>SKGLEDSSTISFITWNIDGLDGCNLPERARGVCSCLALYSPDVVFLQEVIPPYCAYLKKRAASYTIITGNEEGYFTAILLKKGRVKFKSQEIIPFPNTKMMRNLLCVNVSLGGNEFCLMTSHLESTREHSAERIRQLKTVLGKMQEAPDSTTVIFA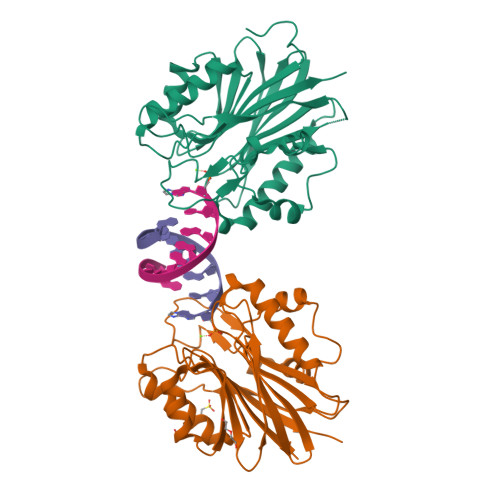GDTNLRDQEVIKCGGLPDNVFDAWEFLGKPKHCQYTWDTKANNNLRIPAAYKHRFDRIFFRAEEGHLIPQSLDLVGLEKLDCGRFPSDHWGLLCTLNVVL[2x]Members of the dynamin family are large GTPases that couple nucleotide hydrolysis to membrane remodelling. Here, we show by sequence analysis and X-ray crystallography that LeoA is a bacterial dynamin-like protein (DLP). Here, we present data demonstrating that the leoABC genes, encoded within a pathogenicity island from enterotoxigenic Escherichia coli (ETEC) strain H10407, are dynamin-like proteins. This is important because LeoA has previously been linked with the secretion of heat labile enterotoxin (LT) through membrane vesicle (MV) biogenesis and release from the bacterial cell surface. Bacterial DLPs (BDLPs) share many of the qualities exhibited by eukaryotic DLPs—they polymerise, exhibit GTPase activity and assemble on lipid into filaments.

Monoclinic crystals of the protein in nucleotide-free state were obtained and the structure solved to 2.7 Å. The crystal structure of LeoA reveals a fold with all the hallmarks of a DLP including the key structural GTPase, neck/BSE and trunk/stalk domains (Figure 2ABC & 3AB). Helix 1 and Helix 2 at the N-terminus form an extended helix-turn-helix motif as observed in BDLP1, that along with Helix 12 and Helix 22 at the C-terminus bundle to form the neck domain. Within the GTPase domain, which is an extended form of the canonical Ras GTPase domain (but smaller than that of BDLP1 by three beta strands), Helix 8 is significantly longer than the equivalent region in human dynamin 1 but similar to that observed in BDLP1. The LeoA trunk domain clearly shares the dynamin canonical fold as observed in other DFMs, and includes a putative hydrophobic membrane binding/paddle domain. Consistent with this, the trunk of LeoA is oriented orthogonal to Helix 12 in the neck, a conformation not observed previously. This 90° kink between trunk Helix 13 and neck Helix 12 is mediated by Gly274 (inset) and represents the equivalent of Hinge 1a in BDLP1. After superimposing the GTPase domain of LeoA upon that of BDLP1 (apo and GDP-bound) and human dynamin 1 (apo), the LeoA trunk is observed to be fully extended, pointing in an opposing direction to the nucleotide binding pocket of the GTPase domain, and yields a ‘flattened’ conformation that is more reminiscent of human guanylate-binding protein 1 (hGBP1). Although this contradicts previous findings, it is consistent with the nucleotide-binding pocket of the GTPase domain being occluded in the LeoA crystal structure. Crystal packing analysis did not reveal any obvious physiologically relevant interactions of LeoA monomers with each other.

> MEQFKQFSIEKQAAINSLLQLRGMLEMLGEMGINISDDLQKVTSAINAIESDVLRIALLGAFSDGKTSVIAAWLGKVMDDMNISMDESSDRLSIYKPEGLPDQCEIVDTPGLFGDKEREVDGRLVMYEDLTRRYISEAHLIFYVVDATNPLKESHSDIVKWVLRDLNKLSSTIFVINKMDEVTSLTDQALFDEQAAIKKANLKGKLQRAADLTAQECEQLNIVCVASNPNGRGLTYWFTKPEHYESRSRINDLKNAATEILKTNVPEVLLVKTGMDVVKDIVIQRVTLASRHLDELNTFVEKNDEDMHRFSNDIKQSRIEVKRLAGELFEELNLMEKQLMSQLRPLDLDDIRPFMDDELGYTEDGVGFKLHLRIKQSVDRFFEQSTAVSQRLSDDITRQLSSSESFLSGLGEGAFRSLGGAFKGVSKISPATLKTTILAARDTIGKLTGYVYKFKPWEATKLAGSIAKWAGPVGAAFTIGSDLWDAYKAHEREQELKEVKASLAKIIKEPFEDIYDVLSSDEKMFAFFAPQIQQMEQVVTELAEKSQAIRDNRQKLSLIQTQLAQLMVPATENHTAR>QTEQGANISDQWTGSELPLAFASDSNPSDPVSNVNDKLISYNNQPANRWTNWNRSNPEASVGVLFGDSGILSKRSVDNLSVGFHEDHGVGAPKSYVIEYYVGKTVPTAPKNPSFVGNEDHVFNDSANWKPVTNLKAPAQLKAGEMNHFSFDKVETYAIRIRMVKADNKRGTSITEVQIFAKQV[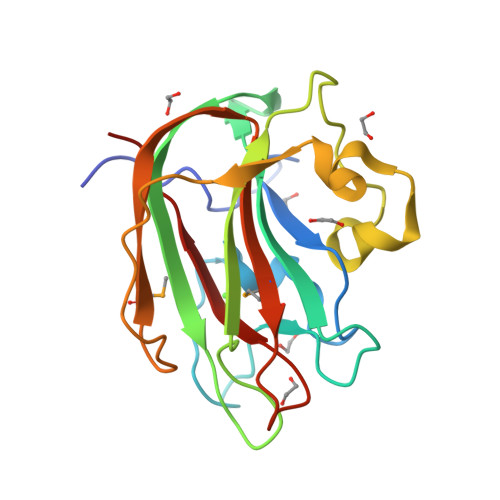2x]> MVKVDLESKRYGEKLKEVFLMLDNNVVECIKEITESSRNGKLVFFVGAGVSTLSDYPQWWRLVDKYHEELYGSPKKGNYSSDEYLRIPQIFYNVKGEMAFDGILKDFFQVDKPTNPIHDKILAMNPAHVITTNYDNLIDTACWKRGKYFSVISAEEDVANATSSRYLLKVHGDFRKGFKGENVVLKEDDYLNYDQNYPLISNLMKTIIATHTIVFIGYGLGDYNINMLLNWVRKLQKDSFHKPFFIRTDPSPIENETLIYYENKGLRIIDAASLIDSNEYDYLERYSAVMDLLIESQENKFITKDDEVIDYIYGKISPLFALQYIRKIDLKHVFEYDYHFEVNGTVVRHKNKGFGYMERFFELKESCDERSKLSKKQYERFNALFNFFEKNGVICMAKDAGTLNTSIEINSLAYHGKYDVMKKFIEEQSVSIEDDYKKAFFLACLGRWEESYDLYSNIILNSIDESNGCVYYLSQINRYRIYQSITQAVTQFNGLGLLTFGRHYKPFTDEFLARIEREMTNFNIDDLFNGMPFEFQKKYKILEFLSDNQFLYDDTVKLFELTNKVRSEMSEGSYSFGMSSDIVVLLRLYDNLRFLYENCLWSVSFHEFHQYIRNSMSLLIEKAEYERTRDIDELGFSFFGKKSGFFMEYYDFVNISRHFKIDDIKNLERSCSIDKIRFGEQEKIEEYLVGIAEEITKQFSANGMNVVFYTQFISEAKAALYFAKYVKLSEEGLGKIVKALLFYFPERDLDIGKRYVWLERLTKCNELPKSIISIIDDFLVLQAEKHIDQNYSEVSSNGLYSRDYGALIKHFEKNFISKRLSEITLCLTQDKQKQIDFLFKLLPLLSTNAKSHLLSFKSVENINDLMNGIRIGLIDEFTPEHEELI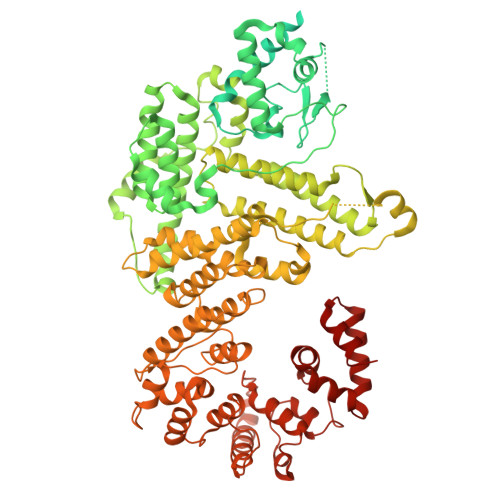IEYLETRKVNYIVEKEKGIQTFSSNDYMSTFGIWYFLEEINNSKMEEFIGMDDQYDFFVDPENFDYKKFIPSWLKNYNDKLLGKIAGNKHMKHHVIEVLKERVKNSNDKRYLEILMNYFI> MASMSETSCDLQATNYIRGCQSKTYDGKIFPGKGGEKQWICKDTIIHGDTNGACIPPRTQNLCVGELWDKSYGGRSNIKQDTKELLKEKIKNAIHKETELLYEYHDTGTAIISKNDKKGQKGKNDPNGLPKGFCHAVQRSFIDYKNMILGTSVNIYEHIGKLQEDIKKIIEKGTPQQKDKIGGVGSSTENVNAWWKGIEREMWDAVRCAITKINKKNNNGIFNGDECGVSPPTGNDEDQSVSWFKEWGEQFCIERLRYEQNIREACTINGKNEKKCINSKSGQGDKIQGACKRKCEKYKKYISEKKQEWDKQKTKYENKYVGKSASDLLKENYPECISANFDFIFNDNIEYKTYYPYGDYSSICSCEQVKYYKYNNAEKKNNKLLCYEKDNDMTWSKKYIKKLENGRSLEGVYVPPRRQQLCLYELFPIIIKNEEGMEKAKEELLETLQIVAEREAYYLWKQYNPTGKGIDDANKKACCAIRGSFYDLEDIIKGNDLVHDEYTKYIDSKLNEIFGSSDTNDIDTKRARTDWWENEAITNGPDRKTIRQLVWDAMQSGVRYAVEEKNENFPLCMGVEHIGIAKPQFIRWLEEWTNEFCEKYTKYFEDMKSKCDPPKRADTCGDNSNIECKKACANYANWLNPKRIEWNGMSNYYNKIYRKSNKESEGGKDYSMIMAPTVIDYLNKRCHGEINGNYICCSCKNIGAYQTTSGTVNKKLQKKETECEEEKGPLDLMNEVLNKMHHHHHH

Pregnancy-associated malaria (PAM) results from the accumulation of PEs in the placenta via attachment to the glycosaminoglycan chondroitin sulphate A (CSA) present in the intervillous spaces. VAR2CSA is the only member of the PfEMP1 family that has been associated with PAM56. The extracellular region of VAR2CSA comprises six DBL domains (type ε or unknown (X)) and a CIDR (CIDRpam) module arranged in the following configuration: DBL1X-DBL2X-CIDRpam-DBL3X-DBL4ε-DBL5ε-DBL6ε. Here we report the crystal structure of the DBL3X-DBL4ε double domain from the FCR3 strain.

The structure was solved and refined at 2.9 Å resolution. The polypeptide chain of the refined structure could be traced from S1218 to V1922 with gaps Q1386-T1398 (DBL3X), N1479-K1485 (DBL3X), G1492-Q1493 (DBL3X), E1614-R1617 (DBL4ε), A1746-G1750 (DBL4ε), D1822-N1835 (DBL4ε), N1871-S1881 (DBL4ε) and N1923-M1950 (DBL4ε). Both domains display the helical secondary structure and the pattern of canonical cysteines characterizing the DBL motif. The double domain forms a compact structure with a short linker (interdomain) region connecting the two DBL modules. The DBL3X-DBL4ε interface is extensive and includes 18 polar interactions between residues that are largely conserved in sequence. A total surface accessible area of 1340 Å2 is buried at the interface between DBL3X and DBL4ε. Contacts between the DBL3X and DBL4ε domains in the crystal structure are made essentially by invariant or highly conserved residues, suggesting that these also occur in the full-length protein and contribute to its compact organization. Subdomain 2 contains the conserved four-helix bundle (αH2, αH3, αH4 and αH5) but, unlike other DBL domains, αH5 possesses an 11-residue insertion (N1744-K1754). The canonical Cys(-1)-Cys(5a) disulfide bridge, linking subdomains 1 and 2 of PfEMP1-DBL domains, is absent in FCR3-DBL4ε structure; this absence is characteristic of the DBL4ε-VAR2CSA domain in other VAR2CSA variants. A novel disulfide bridge, however, is observed between C1689 and C1906, connecting Subdomains 1 and 2 of DBL4ε-FCR3. In DBL4ε-FCR3, however, the interval between the conserved tryptophan residues comprises 18 amino acids (WWX18W), of which 11 form a loop with no regular secondary structure.> MPREVEPSLSERQFVLQALQEGLRLDGRQLDQYRPLSLTFGDQYGVADVTFGKTRVLAKASAEVTVPYADRPLDGIFTIATELSPMTSPTFEVNRPTETEVLLSRLLEKTIRR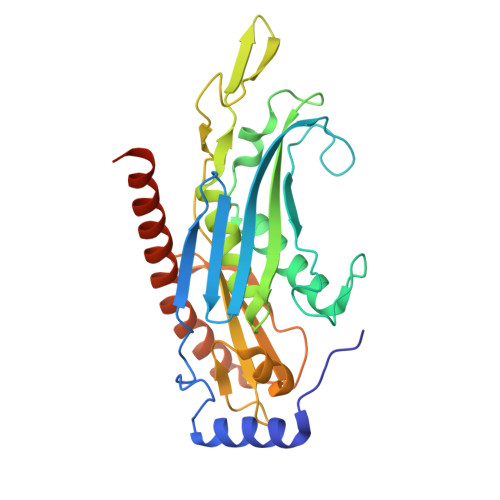SGALDTESLCLVAGQKCWSIRVDVHVMSHDGNLVDAACIAVVAALRHFRKPDTSIESGVLTIYTPAEREPVPLSWLHTPFCVTWSFFGDEGEIAVLDATWLEEQVRVGSCTISMNKHGEICQIAKLGGTPVEAVSLLQCTSIALTKVKEFSDLVDKKLAEDFKRRNPGGLLKELKAENDR>[4x]HMMKGFAMLSIGKVGWIEKEKPAPGPFDAIVRPLAVAPCTSDIHTVFEGAIGERHNMILGHEAVGEVVEVGSEVKDFKPGDRVVVPAITPDWRTSEVQ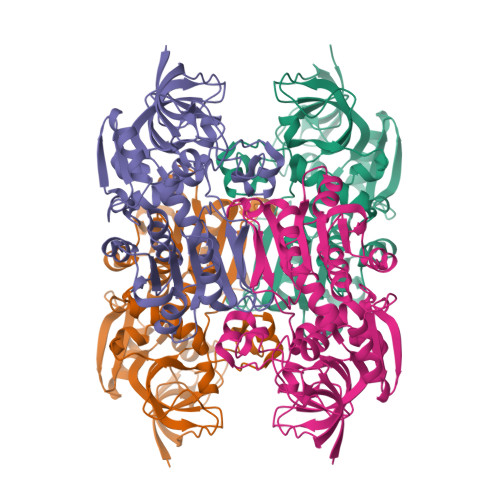RGYHQHSGGMLAGWKFSNVKDGVFGEFFHVNDADMNLAHLPKEIPLEAAVMIPDMMTTGFHGAELADIELGATVAVLGIGPVGLMAVAGAKLRGAGRIIAVSKPPVCVDAAKYYGATDIVNVKDGPIESQIMNLTEGKGVDAAIIAGGNADIMATAVKIVKPGGTIANVNYFGEGEVLPVPRLEWGCGMAHKTIKGGLCPGGRLRMERLIDLVFYKRVDPSKLVTHVFRGFDNIEKAFMLMKDKPKDLIKPVVILA>[2x]GTSTQTKAGSLTIVGTGIESIGQMTLQALSYIEAAAKVFYCVIDPATEAFILTKNKNCVDLYQYYDNGKSALNTYTQMSELMVREVRKGLDVVGVFYGHPGVFVNPSHRALAIAKSEGYRARMLPGVSAEDCLFADLCIDPSNPGCLTYEASDFL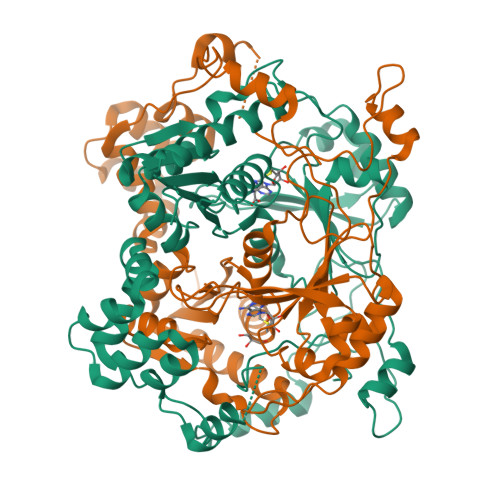IRDRPVSIHSHLVLFQVGCVGIADFNFTGFDNNKFGVLVDRLEQEYGAEHPVVHYIAAMMPHQDPVTDKYTVAQLREPEIAKRVGGVSTFYIPPKARKASNLDIIRRLELLPAGQVPDKKARIYPANQWEPDVPEVEPYRPSDQAAIAQLADHAPPEQYQPLATSKAMSDVMTKLALDPKALADYKADHRAFAQSVPDLTPQERAALELGDSWAIRCAMKNMPSSLLDAARESGEEASQNGFPWVIVVGVIGVIG> EQMC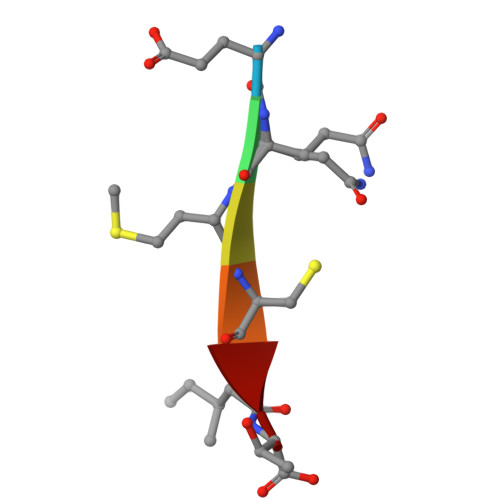IT>[2x]HHHHHHMKLQQLRYIVEVVNHNLNVSSTAEGLYTSQPGISKQVRMLEDELGIQIFARSGKHLTQVTPAGQEIIRIAREVLSKVDAIKSVAGEHTWPDKGSLYIATTHTQARYALPGVIKGFIERYPRVSLHMHQGSPTQIAEAVSKGNADFAIATEALHLYDDLVMLPCYHWNRSIVVTPDHPLAATSSVTIEALAQYPLVTYTFGFTGRSELDTAFNRAGLTPRIVFTATDADVIKTYVRLGLGVGV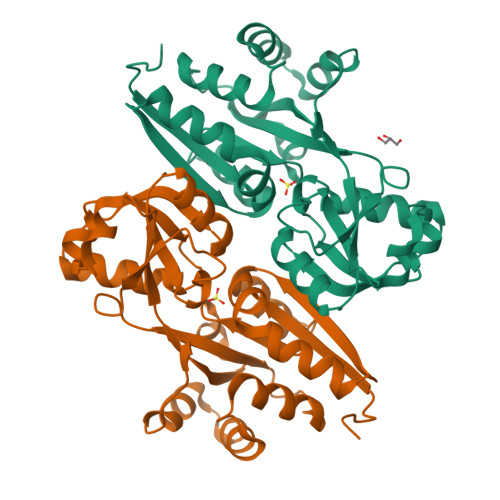IASMAVDPLADPDLVRIDAHDIFSHSTTKIGFRRSTFLRSYMYDFIQRFAPHLTRDVVDTAVALRSNEEIEAMFQDIKLPEK> TDPRAKWVPQDNDIQACDYWRHCSIDGNICDCSGGSLTNCPPGTKLATASWVASCYNPTDGQSYLIAYRDCCGYNVSGRCPCLNTEGELPVYR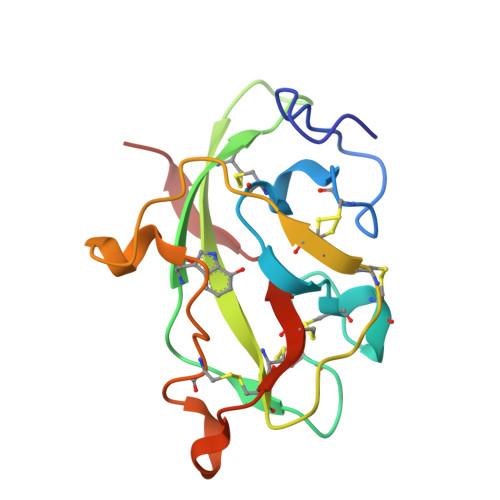PEFANDIIWCFGAEDDAMTYHCTISPIVGKAS> PISPIETVPVKLKPGMDGPKVKQWPLTEEKIKALVEICTEMEKEGKISKIGPENPYNTPVFAIKKKDSTKWRKLVDFRELNKRTQDFWEVQLGIPHPAGLKKKKSVTVLDVGDAYFSVPLDEDFRKYTAFTIPSINNETPGIRYQYNVLPQGWKGSPAIFQSSMTKILEPFKKQNPDIVIYQYMDDLYVGSDLEIGQHRTKIEELRQHLLRWGLTTPDKKHQKEPPFLWMGYELHPDKWTVQPIVLPEKDSWTVNDIQKLVGKLNWASQIYPGIKVRQLCKLLRGTKALTEVIPLTEEAELELAENREILKEP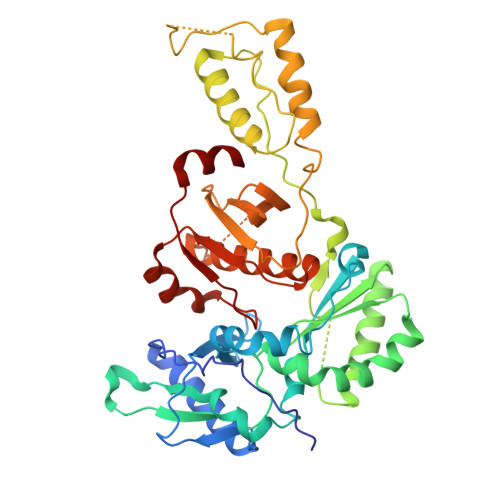VHGVYYDPSKDLIAEIQKQGQGQWTYQIYQEPFKNLKTGKYARMRGAHTNDVKQLTEAVQKITTESIVIWGKTPKFKLPIQKETWETWWTEYWQATWIPEWEFVNTPPLVKLWYQ>[6x]MIPVTELRYFADTQPAYRILKPWWDVFTDYISIVMLMIAVFGGTLQVTQDKMICLPCKWVTKDSCNDSFRGWAASSPEPTYPNSTVLPTPDTGPTGIKYDLDRHQYNYVDAVCYENRLHWFAKYFPYLVLLHTLIFLACSNFWFKFPRTSSKLEHFVSILLKCFDSPWTTRALSETVVEESDPKPAFSKMNGSMDKKSSTVSEDVEATVPMLQRTKSRIEQGIVDRSETGVLDKKEGEQAKALFEKVKKFRTHVEEGDIVYRLYMRQTIIKVIKFALIICYTVYYVHNIKFDVDCTVDIESLTGYRTYRCAHPLATLFKILASFYISLVIFYGLICMYTLWWMLRRSLKKYSFESIREESSYSDIPDVKNDFAFMLHLIDQYDPLYSKRFAVFLSEVSENKLRQLNLNNEWTLDKLRQRLTKNAQDKLELHLFMLSGIPDTVFDLVELEVLKLELIPDVTIPPSIAQLTGLKELWLYHTAAKIEAPALAFLRENLRALHIKFTDIKEIPLWIYSLKTLEELHLTGNLSAENNRYIVIDGLRELKRLKVLRLKSNLSKLPQVVTDVGVHLQKLSINNEGTKLIVLNSLKKMVNLTELELIRCDLERIPHSIFSLHNLQEIDLKDNNLKTIEEIISFQHLHRLTCLKLWYNHIAYIPIQIGNLTNLERLYLNRNKIEKIPTQLFYCRKLRYLDLSHNNLTFLPADIGLLQNLQNLAVTANRIEALPPELFQCRKLRALHLGNNVLQSLPSRVGELTNLTQIELRGNRLECLPVELGECPLLKRSGLVVEEDLFSTLPPEVKERLWRADKEQASNSLEVLFQ

SWELL1 or LRRC8a (leucine-rich repeat-containing protein 8a) encodes a transmembrane protein first described in 2003 as the site of a balanced translocation in an immunodeficient child with agammaglobulinemia and absent B-cells. So, for about a decade, SWELL1 was considered a membrane protein that regulates PI3K-AKT mediated lymphocyte function, and it was not until 2014 that SWELL1/LRRC8a was discovered to also form an essential component of the volume-regulated anion channel (VRAC), forming hetero-hexamers with LRRC8b-e22,23. We previously showed SWELL1 to mediate insulin-PI3K-AKT signaling in adipocytes, skeletal muscle, and endothelium via non-conductive signaling mechanisms. Also, we and others showed SWELL1-LRRC8 channel activity (conductive signaling) in the pancreatic β-cell is required for normal insulin secretion.

As anticipated, SN-403, SN-406, and SN-407 had increased ICl,SWELL inhibitory activity compared to SN-401, with SN-406 and SN-407 having IC50 of 3.1 and 1.6 μM, respectively, and SN-401 IC50 = 3.9 μM. Overexpressing a SWELL1 mutant in WT HEK cells wherein the endogenous SWELL1 R103 is replaced with an electronegative E103 (R103E-SWELL1) functioned as a partial dominant negative for ICl,SWELL current, reducing ICl,SWELL 84%. This residual current in R103E-SWELL1 expressing cells is less sensitive to both SN-401 and SN-407 inhibition, as demonstrated by a rightward shift in the IC50 of SN-401 from 3.9 to 6.0 μM, and SN-407 from 1.6 to 4.2 μM. In initial maps using sixfold symmetry, SN-407 density was less apparent than for DCPIB/SN-40131, potentially due to a reduction in SN-407 occupancy that is a consequence of lower compound solubility or the presence of multiple drug poses in different particles. Pose 1 shows the drug oriented vertically in the channel’s selectivity filter in a manner that is similar to that observed for DCPIB/SN-401, but with the lengthened carboxylate chain coiling to maintain its interaction with R103. In Pose-2, SN-407 is tilted off the SWELL1 central axis, positioning its cyclopentyl group closer to the hydrophobic cleft between SWELL1 subunits. These data confirm lengthening the carboxylate chain in SN-407 preserves electrostatic interactions with R103 and enables additional contacts between the carboxylate chain and upper hydrophobic moieties in distinct binding poses, consistent with the results of our docking simulations. However, collectively, these molecular docking, cryo-EM, and functional experiments indicate that SN-401 and SWELL1-active congeners (SN-403/406/407) bind to SWELL1-LRRC8 hexamers at both R103 (via carboxylate end) and at the interface between adjacent LRRC8 monomers (via hydrophobic end), to potentially stabilize the closed state of the channel, and thereby inhibit ICl,SWELL activity. Indeed, SN-401/SN-407 cryo-EM data and molecular docking simulations likely reflect the closed state of the SWELL1 homomer.>[2x]SNAMADWVTGKVTKVQNWTDALFSLTVHAPINPFTAGQFTKLGLEIDGERVQRAYSYVNAPDNPNLEFYLVTVPQGKLSPRLAALKPGDEVQVVSDASGFFVLDEVPDCETLWMLATGTAIGPYLSILQYGQDVARFKNLVLVHAARFAADLSYLPLMLELQQRYEGKLRIQTV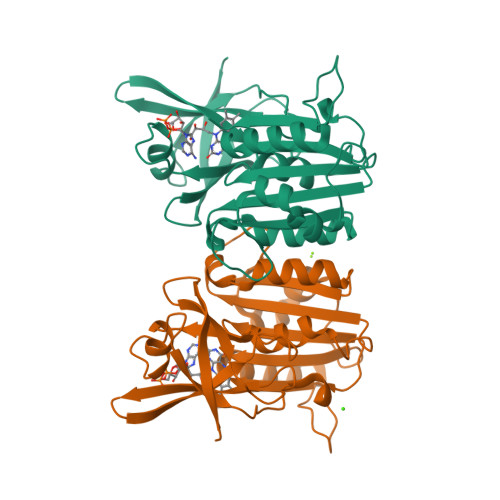VSRENVPGSLTGRVPALIENGELEKAVGLPMDKETSHVMLCGNPQMVRDTQQLLKETRQMTKHLRRRPGHMTAEHYW> MGHKKNGHRRQIKERENQNKFERSTYTNNAKN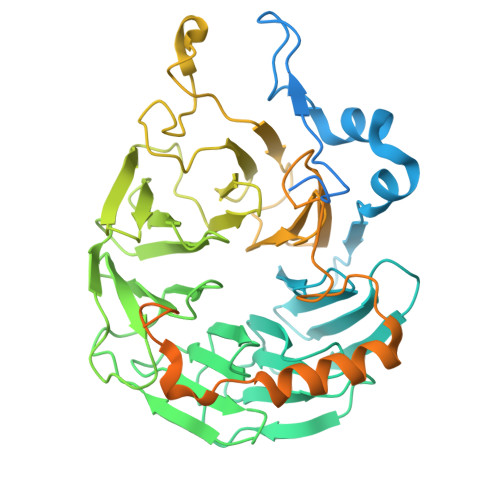NHTQTKDKKLRAGLKKIDEQYKKAVSSAAATDYLLPESNGYLEPENELEKTFKVQQSEIKSSVDVSTANKALDLSLKEFGPYHIKYAKNGTHLLITGRKGHVASMDWRKGQLRAELFLNETCHSATYLQNEQYFAVAQKKYTFIYDHEGTELHRLKQHIEARHLDFLPYHYLLVTAGETGWLKYHDVSTGQLVSELRTKAGPTMAMAQNPWNAVMHLGHSNGTVSLWSPSMPEPLVKLLSARGPVNSIAIDRSGYYMATTGADRSMKIWDIRNFKQLHSVESLPTPGTNVSISDTGLLALSRGPHVTLWKDALKLSGDSKPCFGSMGGNPHRNTPYMSHLFAGNKVENLGFVPFEDLLGVGHQTGITNLIVPGAGEANYDALELNPFETKKQRQEQEVRTLLNKLPADTITLDPNSIGSVDKRSSTIRLNAKDLAQTTMDANNKAKTNSDIPDVKPDVKGKNSGLRSFLRKKTQNVIDERKLRVQKQLDKEKNIRKRNHQIKQGLISEDHKDVIEEALSRFG>XGQLEEIAKQLQQIAWQL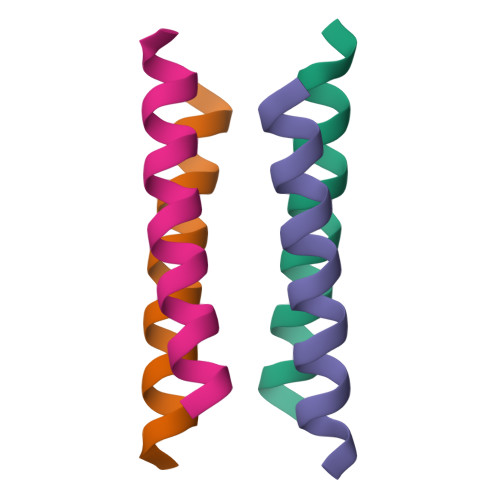KKIAQGX[2x]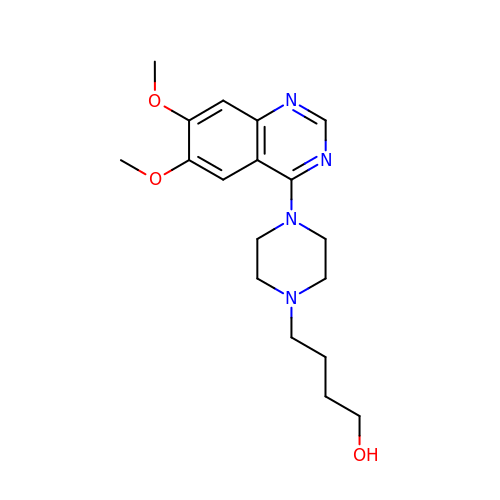4-[4-(6,7-dimethoxyquinazolin-4-yl)piperazin-1-yl]butan-1-ol | C18 H26 N4 O3 | AUJDIJFFUZNFMZ-UHFFFAOYSA-N>MRDLKGIFSALLVSFNEDGTINEKGLRQIIRHNIDKMKVDGLYVGGSTGENFMLSTEEKKEIFRIAKDEAKDQIALIAQVGSVNLKEAVELGKYATELGYDCLSAVTPFYYKFSFPEIKHYYDTIIAETGSNMIVYSIPFLTGVNMGIEQFGELYKN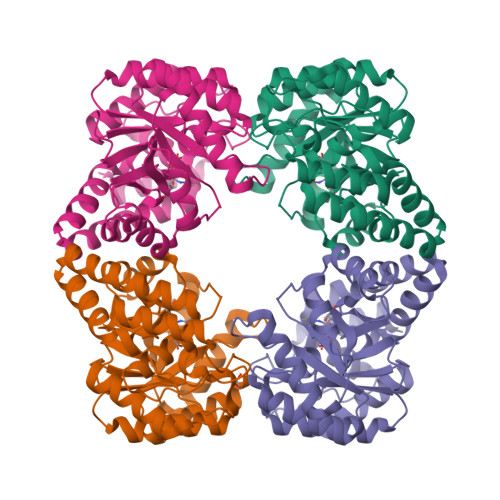PKVLGVKFTAGDFYLLERLKKAYPNHLIWAGFDEMMLPAASLGVDGAIGSTFNVNGVRARQIFELTKAGKLKEALEIQHVTNDLIEGILANGLYLTIKELLKLEGVDAGYCREPMTSKATAEQVAKAKDLKAKFLS[4x]>[4x]GSPASGTSLSAAIHRTQLWFHGRISREESQRLIGQQGLVDGLFLVRESQRNPQGFVLSLCHLQKVKHYLILPSEEEGRLYFSMDDGQTR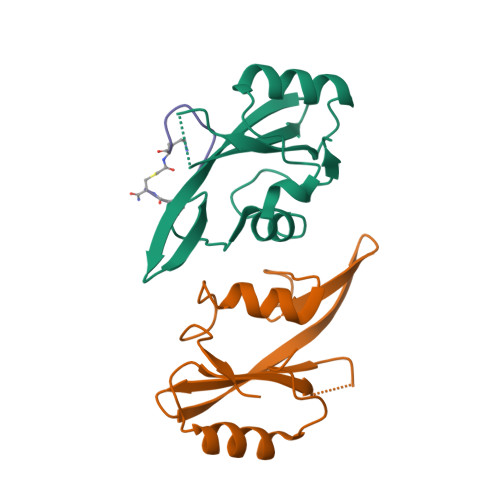FTDLLQLVEFHQLNRGILPCLLRHCCTRVAL;>[2x]KFEGYDNEFPX> MARARGRGRRDLKSEINIVPLLDVLLVLLLIFMATAPIITQSVEVDLPDATESQAVSSNDNPPVIVEVSGIGQYTVVVEK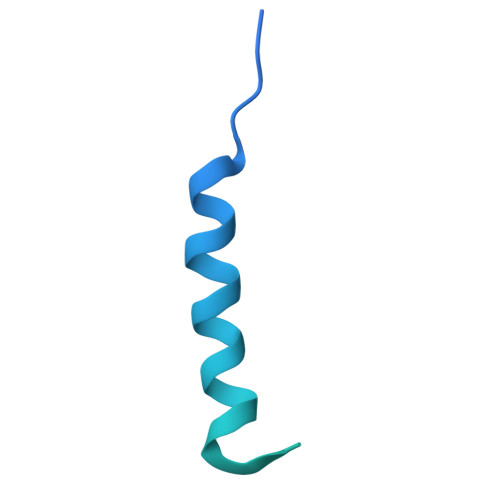DRLERLPPEQVVAEVSSRFKANPKTVFLIGGAKDVPYDEIIKALNLLHSAGVKSVGLMTQPI> MVRGSRPSGGQAGSRHFLGGVDGQCYAGCLSTESRMAKGKLVLGLDIGSTSIKMILLKEQRKRGEVIYALQSFGMKPLPPEAIVDGALMNSTAIVQAVQDLMSELKVKGKDVAIGVSGHSVIIKKIQMPRMSQDELEESIQWEAEQYIPFDVKDVNIDTQILDGGGNDATGQMDVLLVA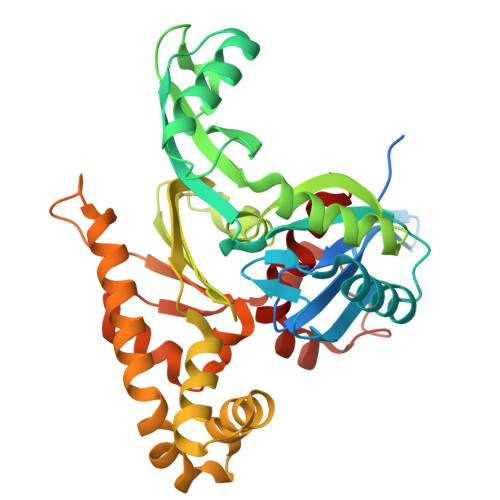AKKDMINDYTTVVSEAGLAPVVVDVDAFAVQNMFSVNYDVPERETVVLINAGASVVNINIISNGATVFTRDVTIGGNQFTEEIQKQLNVSYEEAEALKIGGNGADADAVVPQDVERVLSSVAEQVAGEIQRSLDFYAGTAADSNFSKVYLSGGTAKIPALFKTIEARTGVPVEILNPFRKIEVDNRKFDPAFVMDVAPMAAVAVGLALRRPGDKLA4-cyano-N-(2-cyclohex-1-en-1-yl-4-piperidin-4-ylphenyl)-1H-imidazole-2-carboxamide 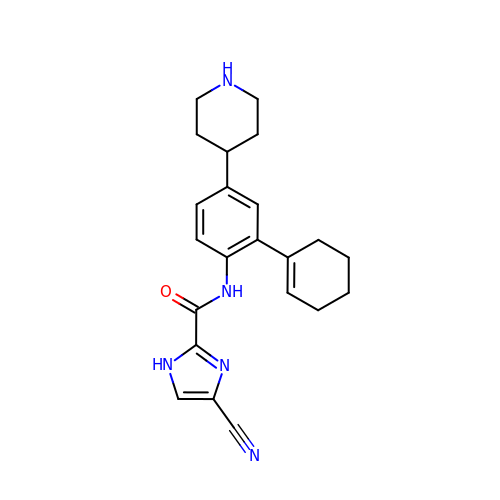| C22 H25 N5 O | XPCQXAQALLRVJQ-UHFFFAOYSA-N Semaphorins transduce signal through the plexin receptors, which are single-pass transmembrane proteins localized on the cell surface. Ectromelia virus secrets a protein named A39R that is a Sema7A mimic. The class C plexin PlexinC1 is unique in that it only has two PSI and four IPT domains in the extracellular region, rather than three and six, respectively, in classes A, B, and D plexins. Structural analyses have shown that a dimeric semaphorin binds two plexin molecules through interactions mediated by their respective Sema domains, supporting the ligand-induced dimerization model for plexin activation.

To address these questions, we purified full-length human PlexinC1 and reconstituted the 2:2 dimeric active complex with its high affinity ligand A39R from ectromelia virus. We determined the structure of the complex to 2.9 Å resolution by using cryo-electron microscopy (Cryo-EM). We then reconstituted the complex into peptidisc, a recently developed short peptide that can stabilize the transmembrane region of membrane proteins in the absence of detergent. The cryo-EM structure of full-length PlexinC1/A39R complex shows that the pair of the Sema domain in the A39R dimer bind two protomers of PlexinC1 at two opposite sides, as seen in all the crystal structures of plexin/semaphorin complexes reported previously. The overall architecture of PlexinC1 extracellular region appears quite different from the ring-shape of class A plexins. The Sema and IPT2 domains in PlexinC1 make an extensive inter-domain interface. In particular, Cys412 in blade-6 of the Sema domain and Cys703 in the C–C′ loop of IPT2 form a disulfide bond to covalently link the two domains. The cryo-EM structure of the full-length PlexinC1/A39R shows similar convergence of the two membrane-proximal IPT4 domains from the two PlexinC1 protomers. However, due to the different architecture of its extracellular region as compared with class A plexins, the two copies of the IPT4 domain are arranged in an antiparallel fashion (See details below). Our structure shows that while the β-sandwiches of the two IPT4 protomers in the dimeric complex face to each other closely, they do not make any direct contact.

>[2x]ELEIEWHKFETSEEIISTYLIDDVLYTGVNGAVYTFSNNELNKTGLTNNNNYITTSIKVEDTLVCGTNNGNPKCWKIDGSEDPKYRGRGYAPYQNSKVTIISHNECVLSDINISKEGIKRWRRFDGPCGYDLYTADNVIPKDGVRGAFVDKDGTYDKVYILFTDTIDTKRIVKIPYIAQMCLNDEGGPSSLSSHRWSTFLKVELECDIDGRSYRQIIHSKAIKTDNDTILYVFFDSPYSKSALCTYSMNAIKHSFSTSKLGGYTKQLPSPAPGICLPAGKVVPHTTFDIIEQYNELDDIIKPLSQPIFEGPSGVKWFDIKEKENEHREYRIYFIKENTIYSFDTKSKQTRSAQVDARLFSVMVTSKPLFIADIGIGVGIPRMKKILKMGTHHHHHHHH;>ADEPVWRSEQAIGAIAASQEDGVFVASGSCLDQLDYSLEHSLSRLYRDQAGNCTEPVSLAPPARPRPGSSFSKLLLPYREGAAGLGGLLLTGWTFDRGACEVRPLGNLSRNSLRNGTEVVSCHPQGSTAGVVYRAGRNNRWYLAVAATYVLPEPETASRCNPAASDHDTAIALKDTEGRSLATQELGRLKLCEGAGSLHFVDAFLWNGSIYFPYYPYNYTSGAATGWPSMARIAQSTEVLFQGQASLDCGHGHPDGRRLLLSSSLVEALDVWAGVFSAAAGEGQERRSPTTTALCLFRMSEIQARAKRVSWDFKTAESHCKEGDQPERVQPIASSTLIHSDLTSVYGTVVMNRTVLFLGTGDGQLLKVILGENLTSNCPEVIYEIKEETPVFYKLVPDPVKNIYIYLTAGKEVRRIRVANCNKHKSCSECLTATDPHCGWCHSLQRCTFQGDCVHSENLENWLDISSGAKKCPKIQIIRSSKEKTTVTMVGSFSPRHSKCMVKNVDSSRELCQNKSQPNRTCTCSIPTRATYKDVSVVNVMFSFGSWNLSDRFNFTNCSSLKECPACVETGCAWCKSARRCIHPFTACDPSDYERNQEQCPVAVEKTSGGGRPKENKGNRTNQALQVFYIKSIEPQKVSTLGKSNVIVTGANFTRASNITMILKGTSTCDKDVIQVSHVLNDTHMKFSLPSSRKEMKDVCIQFDGGNCSSVGSLSYIALPHCSLIFPATTWISGGQNITMMGRNFDVIDNLIISHELKGNINVSEYCVATYCGFLAPSLKSSKVRTNVTVKLRVQDTYLDCGTLQYREDPRFTGYRVESEVDTELEVKIQKENDNFNISKKDIEITLFHGENGQLNCSFENITRNQDLTTILCKIKGIKTASTIANSSKKVRVKLGNLELYVEQESVPSTWYFLIVLPVLLVIVIFAAVGVTRHKSKELSRKQSQQLELLESELRKEIRDGFAELQMDKLDVVDSFGTVPFLDYKHFALRTFFPESGGFTHIFTEDMHNRDANDKNESLTALDALICNKSFLVTVIHTLEKQKNFSVKDRCLFASFLTIALQTKLVYLTSILEVLTRDLMEQCSNMQPKLMLRRTESVVEKLLTNWMSVCLSGFLRETVGEPFYLLVTTLNQKINKGPVDVITCKALYTLNEDWLLWQVPEFSTVALNVVFEKIPENESADVCRNISVNVLDCDTIGQAKEKIFQAFLSKNGSPYGLQLNEIGLELQMGTRQKELLDIDSSSVILEDGITKLNTIGHYEISNGSTIKVFKKIANFTSDVEYSDDHCHLILPDSEAFQDVQGKRHRGKHKFKVKEMYLTKLLSTKVAIHSVLEKLFRSIWSLPNSRAPFAIKYFFDFLDAQAENKKITDPDVVHIWKTNSLPLRFWVNILKNPQFVFDIKKTPHIDGCLSVIAQAFMDAFSLTEQQLGKEAPTNKLLYAKDIPTYKEEVKSYYKAIRDLPPLSSSEMEEFLTQESKKHENEFNEEVALTEIYKYIVKYFDEILNKLERERGLEEAQKQLLHVKVLFDEKKKCKWMGTSSGLEVLFQ[2x]Azoreductases are a related but previously thought to be distinct group of NAD(P)H dependent flavoenzymes that have been identified in a number of species from bacteria, to mammals. In order to help understand the mechanism of quinone reduction by azoreductases the structures of paAzoR1 bound to two quinone substrates (UQ1 and AQN) have been solved via X-ray crystallography. We have shown the azoreductase family are very active NAD(P)H quinone oxidoreductases with broad specificity profiles and as a result they may play an important role in detoxifying the quinones secreted by many of the host organisms of P. aeruginosa. paAzoR1 has a preference for benzoquinones e.g. Bzq.

The structure of paAzoR1 bound to AQN was solved at a resolution of 1.8 Å with final Rfree and Rwork values of 18.5% and 16.2% respectively, while UQ1 was solved at 2.0 Å with final Rfree and Rwork values of 23.6% and 18.5% respectively. In both structures, the quinone is only observed binding to one of the two active sites, although positive difference density is observed in the alternate active sites there was insufficient to unambiguously build in the model. In the structure of paAzoR1 binding to AQN, AQN makes hydrophobic contacts with Phe60, Phe100, Phe120, Tyr131 and Phe173. AQN also forms π-π stacking interactions with the central ring of FMN while the sulphonate group points into a water filled channel. Neither quinone oxygen is in a position to form a hydrogen bond with Asn99 upon reduction as has been previously observed most probably due to the bulky nature of AQN. The binding orientations of UQ1 and AQN differ significantly, with UQ1 binding parallel to the ring system of FMN while AQN binds at almost a 90° angle to FMN. These differing binding orientations correspond to those observed when methyl red binds to either the wild type enzyme in the case of AQN and the Y131F mutant in the case of UQ1. In the case of AQN one would expect the δ+ carbon, which accepts the hydride, to be the carbon attached to the negatively charged sulphate. However the sulphate of AQN is not easily accommodated within the primarily hydrophobic active site of paAzoR1. As a result an unmodified carbon atom accepts the proton in a less favourable reaction possibly contributing to the lower rate of reduction observed of AQN by all azoreductases compared to other quinones.

>[2x]MSRILAVHASPRGERSQSRRLAEVFLAAYREAHPQARVARREVGRVPLPAVTEAFVAAAFHPQPEQRSLAMQADLALSDQLVGELFDSDLLVISTPMYNFSVPSGLKAWIDQIVRLGVTFDFVLDNGVAQYRPLLRGKRALIVTSRGGHGFGPGGENQAMNHADPWLRTALGFIGIDEVTVVAAEGEESGGRSFEDSCDEAEQRLLALARSA> QEITVDEFSNIRENPVTPWNPEPSAPVIDPTAYIDPQASVIGEVTIGANVMVSPMASIRSDEGMPIFVGDRSNVQDGVVLHALETINEEGEPIEDNIVEVDGKEYAVYIGNNVSLAHQSQVHGPAAVGDDTFIGMQAFVFKSKVGNNCVLEPRSAAIGVTIPDGRYIPAGMVVTSQAEADK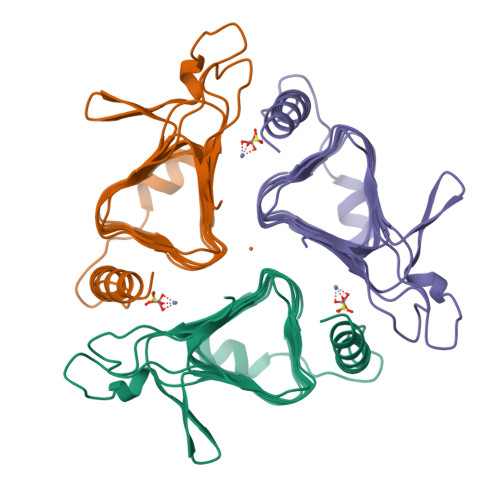LPEVTDDYAYSHTNEAVVAVNVHLAEGYKETS>[6x]MNPVHILAKKGEVAERVLVVGDPGRARLLSTLLQNPKLTNENRGFLVYTGKYNGETVSI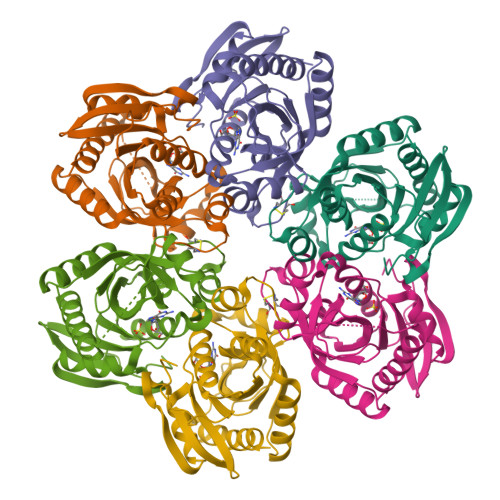ATHGIGGPSIAIVLEELAMLGANVFIRYGTTGALVPYINLGEYIIVTGASYNQGGLFYQYLRDNACVASTPDFELTNKLVTSFSKRNLKYYVGNVFSSDAFYAEDEEFVKKWSSRGNIAVEMECATLFTLSKVKGWKSATVLVVSDNLAKGGIWITKEELEKSVMDGAKAVLDTLTS> GPLSGLKKLIPEEGRELIGSVKKIIKRVSNEEKANEMEKNILKILIKVFFYIDSKAIQIGDLAKVDRALRDGFNHLDRAFRYYGVKKAADLVVILEKASTALKEAEQETVTLLTPFFRPH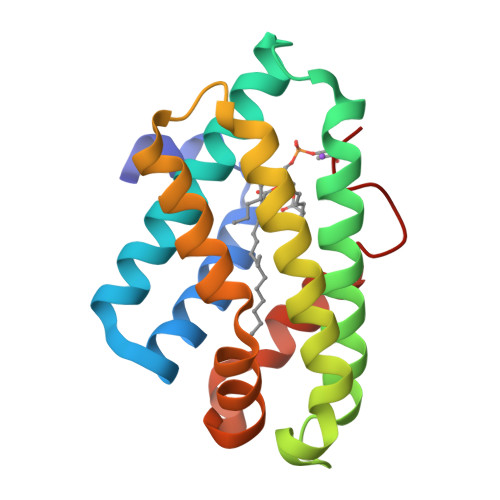NIQLIRNTFAFLGSLDFFTKVWDDLEIEDDLFLLISALNKYTQIELIY> ATSDSNMLLNYVPVYVMLPLGVVNVDNVFEDPDGLKEQLLQLRAAGVDGVMVDVWWGIIELKGPKQYDWRAYRSLLQLVQECGLTLQAIMSFHQCGGNVGDIVNIPIPQWVLDIGESNHDIFYTNRSGTRNKEYLTVGVDNEPIFHGRTAIEIYSDYMKSFRENMSDFLESGLIIDIEVGLGPAGQLRYPSYPQSQGWEFPGIGEFQCYDKYLKADFKAAVARAGHPEWELPDDAGKYNDVPESTGFFKSNGTYVTEKGKFFLTWYSNKLLNHGDQILDEAN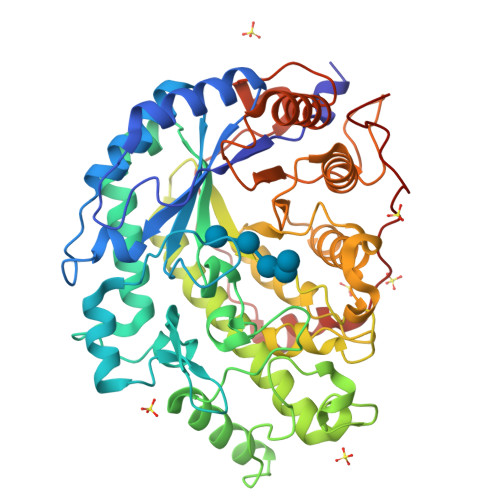KAFLGCKVKLAIKVSGIHWWYKVENHAAELTAGYYNLNDRDGYRPIARMLSRHHAILNFTCLEMRDSEQPSDAKSGPQELVQQVLSGGWREDIRVAGENALPRYDATAYNQIILNARPQGVNNNGPPKLSMFGVTYLRLSDDLLQKSNFNIFKKFVLKMHADQDYCANPQKYNHAITPLKPSAPKIPIEVLLEATKPTLPFPWLPETDMKVDG> GAGAMSSRKKPSRRTRVLVGGAALAVLGAGVVGTVAANAADTTEATPAAAPVAARGGELTQSTHLTLEAATKAARAAVEAAEKDGRHVSVAVVDRNGNTLVTLRGDGAGPQSYESAERKAFTAVSWNAPTSELAKRLAQAPTLKDIPGTLFLAGGTPVTAKGAP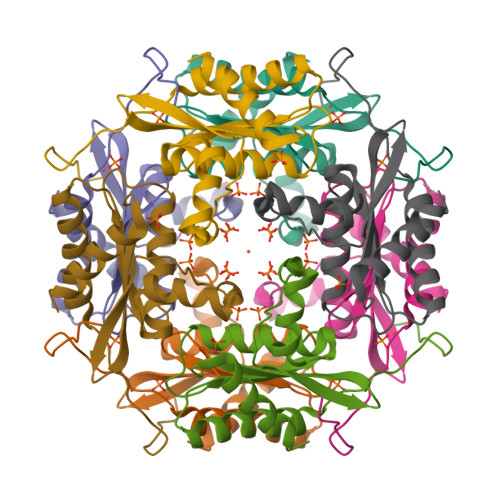VAGIGVAGAPSGDLDEQYARAGAAVLGH> MTQPLVGKQILIVEDEQVFRSLLDSWFSSLGATTVLAADGVDALELLGGFTPDLMICDIAMPRMNGLKLLEHIRNRGDQTPVLVISATENMADIAKALRLGVEDVLLKPVKDLN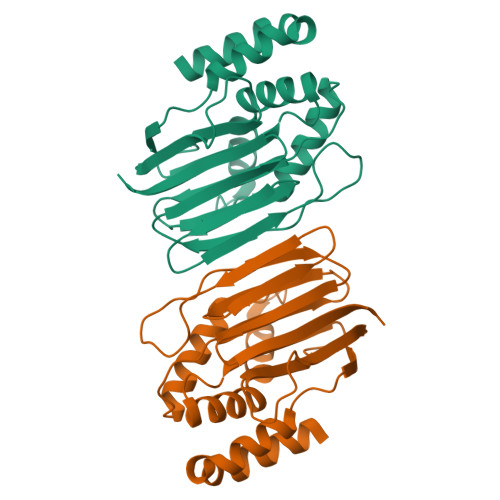RLREMVFACLYPSMFNSRVEEEERLFRDWDAMVDNPAAAAKLLQELQPPVQQVISHCRVNYRQLVAADKPGLVLDIAALSENDLAFYCLDVTRAGHNGVLAALLLRALFNGLLQEQLAHQNQRLPELGALLKQVNHLLRQANLPGQFPLLVGYYHRELKNLILVSAGLNATLNTGEHQVQISNGVPLGTLGNAYLNQLSQRCDAWQCQIWGTGGRLRLMLSAE> AEGTRGRSSTARCSLFGSDFVNTFDGSMYSFAGYCSYLLAGGCQKRSFSIIGDFQNGKRVSL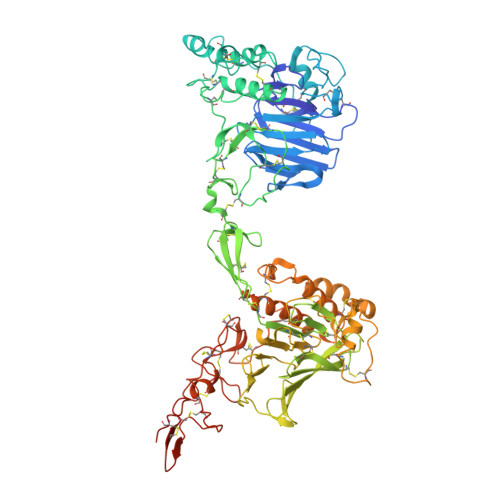SVYLGEFFDIHLFVNGTVTQGDQRVSMPYASKGLYLETEAGYYKLSGEAYGFVARIDGSGNFQVLLSDRYFNKTCGLCGNFNIFAEDDFMTQEGTLTSDPYDFANSWALSSGEQWCERASPPSSSCNISSGEMQKGLWEQCQLLKSTSVFARCHPLVDPEPFVALCEKTLCECAGGLECACPALLEYARTCAQEGMVLYGWTDHSACSPVCPAGMEYRQCVSPCARTCQSLHINEMCQERCVDGCSCPEGQLLDEGLCVESTECPCVHSGKRYPPGTSLSRDCNTCICRNSQWICSNEECPGECLVTGQSHFKSFDNRYFTFSGICQYLLARDCQDHSFSIVIETVQCADDRDAVCTRSVTVRLPGLHNSLVKLKHGAGVAMDGQDVQLPLLKGDLRIQHTVTASVRLSYGEDLQMDWDGRGRLLVKLSPVYAGKTCGLCGNYNGNQGDDFLTPSGLAEPRVEDFGNAWKLHGDCQDLQKQHSDPCALNPRMTRFSEEACAVLTSPTFEACHRAVSPLPYLRNCRYDVCSCSDGRECLCGALASYAAACAGRGVRVAWREPGRCELNCPKGQVYLQCGTPCNLTCRSLSYPDEECNEACLEGCFCPPGLYMDERGDCVPKAQCPCYYDGEIFQPEDIFSDHHTMCYCEDGFMHCTMSGVPGSLLPDAVLSSPLSHRSKR> GSHMEAVQNRIVEAAERVPGVRGVIHLRARYVGQDIWADMIIGVDPENTVEQAAEICEAVQAAVCGKIRRIESLHVSAAAREIG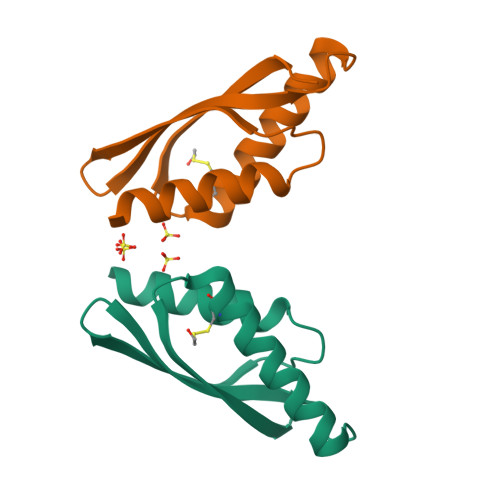DTTKPSFSDQPLSFDEVMLSKVDN>[2x]SDVFHLGLTKNDLQGAQLAIVPGDPERVEKIAALMDKPVKLASHREFTTWRAELDGKPVIVCSTGIGGPSTSIAVEELAQLGI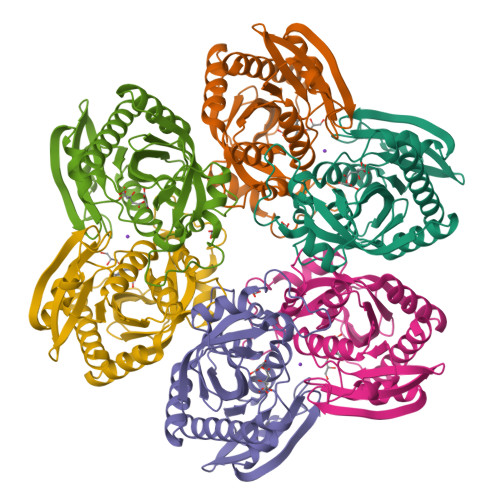RTFLRIGTTGAIQPHINVGDVLVTTASVRLDGASLHFAPLEFPAVADFECTTALVEAAKSIGATTHVGVTASSDTFYPGQERYDTYSGRVVRHFKGSMEEWQAMGVMNYEMESATLLTMCASQGLRAGMVAGVIVNRTQQEIPNAETMKQTESHAVKIVVEAARRLL> EEYVFESPKMKEILEKIKKISCAECPVLITGESGVGKEVVARLIHKLSDRSKEPFVALNVASIPRDIFEAELFGYEKGAFTGAVSSKEGFFELADGGTLFLDEIGELSLE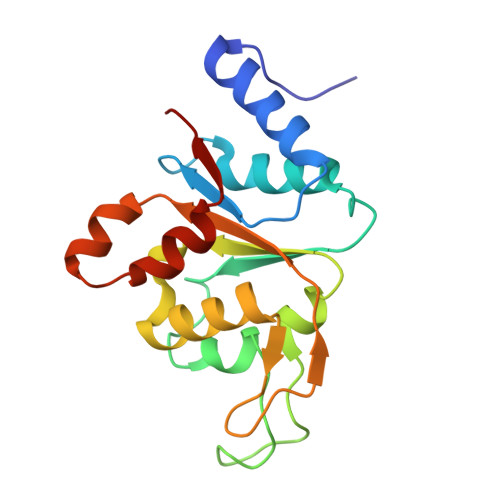AQAKLLRVIESGKFYRLGGRKEIEVNVRILAATNRNIKELVKEGKFREDLYYRLGVIEIEIPP>[3x]ASNFTQFVLVDNGGTGDVTVAPSNFANGVAEWISSNSRSQAYKVTCSVRQSSAQNRKYTIKVEVPKVATQTVGGVELPVAAWRSYLNMELTIPIFATNSDCELIVKAMQGLLKDGNPIPSAIAANSGIY

To prevent this, we describe a method to encapsulate target proteins within highly hydrophilic, structurally homogeneous, and stable protein shells, which we refer to as “nanocrates” for this purpose. Our approach was inspired by the established use of natural virus capsids and engineered protein containers for packaging applications. We adapted this concept for cryo-EM by encapsulating target proteins within symmetric MS2 bacteriophage-derived “nanocrates”. Being highly symmetric, the nanocrates do not adopt a preferred orientation at the AWI, and therefore their enveloped cargoes are randomly oriented. Nanocrate densities can be computationally subtracted during single-particle cryo-EM analysis to allow for high-resolution reconstruction of the molecules inside.

Briefly, we purified MS2 capsids from *E. coli*, performed disassembly in an acidic solvent with the removal of packaged viral RNA by centrifugation, and reassembled the capsid proteins at neutral pH in the presence of ApoF. We designate the reassembled cages as nanocrates (“nc”) to distinguish particles derived from disassembly and reassembly, rather than another commonly used packing strategy in which cargo-containing virus-like particles (VLPs) are derived from simultaneous expression and packaging in the expression host. The @ symbol is used to designate the packaged species. Cryo-EM image analysis of MS2nc@ApoF reassembly showed a mixed population of empty and cargo-filled MS2nc particles (**[Fig fig1]**). From 5,000 micrographs, we selected ∼240,000 particles and used icosahedral symmetry to produce a map of MS2nc at a resolution of 1.86 Å. From a methodological perspective, we found that one could not simply use the published structure of MS2 for the nanocrate density subtraction step. Instead, it was necessary to employ the experimental data for MS2nc obtained for each sample to calculate the shell density for subtraction. The nanocrate thereby provides a built-in resolution standard, determining the principal resolution limit of the dataset. It can also be used to tune dataset processing parameters such as coma, magnification anisotropy, per-particle CTF, Cs value, and pixel size.> MGGSEVGTVPVTWRLGVDVGERSIGLAAVSYEEDKPKEILAAVSWIHDGGVGDERSGASRLALRGMARRARRLRRFRRARLRDLDMLLSELGWTPLPDKNVSPVDAWLARKRLAEEYVVDETERRRLLGYAVSHMARHRGWRNPWTTIKDLKNLPQPSDSWERTRESLEARYSVSLEPGTVGQWAGYLLQRAPGIRLNPTQQSAGRRAELSNATAFETRLRQEDVLWELRCIADVQGLPEDVVSNVIDAVFCQKRPSVPAERIGRDPLDPSQLRASRACLEFQEYRIVAAVANLRIRDGSGSRPLSLEERNAVIEALLAQTERSLTWSDIALEILKLPNESDLTSVPEEDGPSSLAYSQFAPFDETSARIAEFIAKNRRKIPTFAQWWQEQDRTSRSDLVAALADNSIAGEEEQELLVHLPDAELEALEGLALPSGRVAYSRLTLSGLTRVMRDDGVDVHNARKTCFGVDDNWRPPLPALHEATGHPVVDRNLAILRKF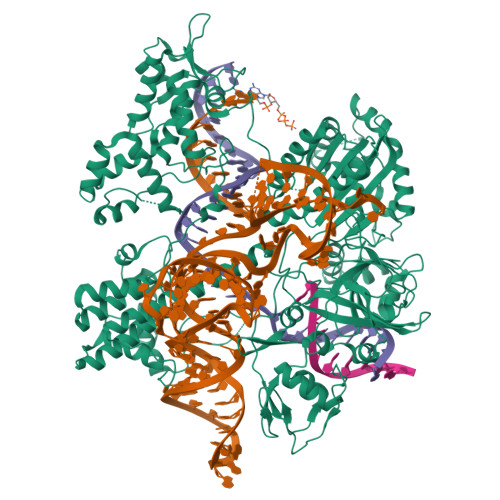LSSATMRWGPPQSIVVELGGGSAGGYAAVALRDRLLSYGEKNGVAQVAVFRGGVTAEARRWLDISIERLFSRVAIFAQSTSTKRLDRRHHAVDAVVLTTLTPGVAKTLADARSRRVSAEFWRRPSDVNRHSTEEPQSPAYRQWKESCSGLGDLLISTAARDSIAVAAPLRLRPTGALHEETLRAFSEHTVGAAWKGAELRRIVEPEVYAAFLALTDPGGRFLKVSPSEDVLPADENRHIVLSDRVLGPRDRVKLFPDDRGSIRVRGGAAYIASFHHARVFRWGSSHSPSFALLRVSLADLAVAGLLRDGVDVFTAELPPWTPAWRYASIALVKAVESGDAKQVGWLVPGDELDFGPEGVTTAAGDLSMFLKYFPERHWVVTGFEDDKRINLKPAFLSAEQAEVLRTERSDRPDTLTEAGEILAQFFPRCWRATVAKVLCHPGLTVIRRTALGQPRWRRGHLPYSWRPWSADPWSTAEL>GSHMIARIIGEIGIEGARFIEENIDEQFKALRYLSKGIDSETFVKLVIANSLVSYQLTGKGEQWWWEFAKYFYGRDVKSIYLAYKEFLPNSRFNRRLIPQKLSRIRRVETFLSTLTEERIEEYYGDMSSLWGSIARALGVDKESKTVVFSVKMFGYAARIVLSTFNPYPMEIP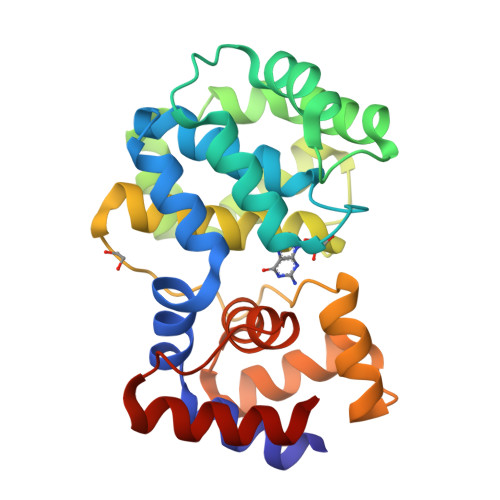IPEDSRIVKLTKKLTNEKPRKFWMKIARESGVPPLHIDSILWPLLGGASIDSAPPELRDKLAELIKIIR[2x]> GDEWTDEQFKQLISFKTQPGGWGVTDVHVRYANSAKYTYNLPVLVSGSTDNTDDRLVSFSLRDDTLDILNFEKFGNRPELYFRELPQKYYSFPKELTIPAGQSHALLPIEFSLDGLDDSQKWALPLKVCEDANGTYAVNPRKYYRTAVLRPILFNEFSGRFSGSSLLGTMAGESDIKFSSTEIKLNVVTDSIVFFYAGQRTEDYEDRINYKVFLQFTGDKVDSKKDLYKMKIWAENEKLK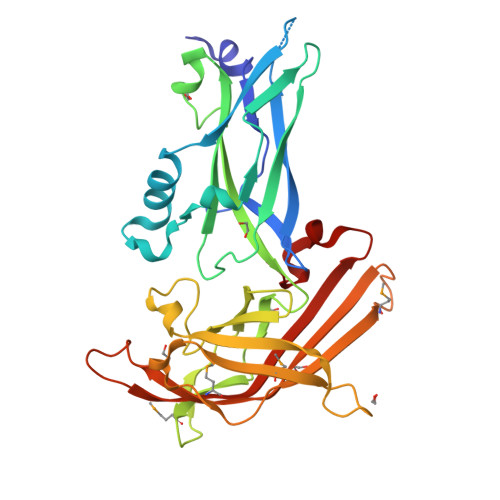FNSYSTPTYKVSSEMDATKTYLKHTYIVISDIDFDFVDYTSVPNYEIEYNMKGGLSVSRDLDTRKPDEDQGSDSKWW(3~{S},3'~{S},4'~{S})-4'-azanyl-6-chloranyl-3'-(3-chlorophenyl)-1'-(2,2-dimethylpropyl)spiro[1~{H}-indole-3,2'-pyrrolidine]-2-one | C22 H25 Cl2 N3 O | 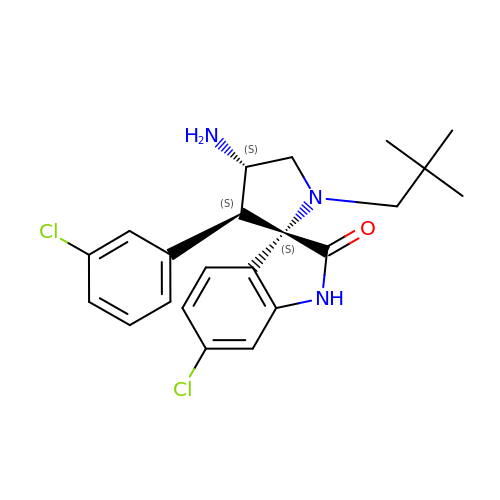CWDGHXCEKKZGEC-ZWCUEREDSA-N>MKYPPSLVSLIRELSRLPGIGPKSAQRLAFHLFEQPREDIERLASALLEAKRDLHVCPICFNITDAEKCDVCADPSRDQRTICVVEEPGDVIALERSGEYRGLYHVLHGVLSPMNGVGPDKLHIKPLLPRVGQGMEVILATGTTVEGDATALYLQRLLEPLGAAI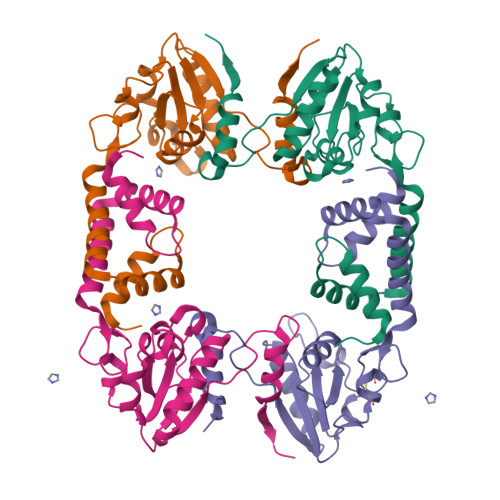SRIAYGVPVGGSLEYTDEVTLGRALTGRQTVSKPQPPQRPGDEDGADGAAVPASRLEHHHHHH[4x]> IDPRFPHHHPRPQSFWEARAKALESLLIEKGHLSSDASERVIKHYEHEL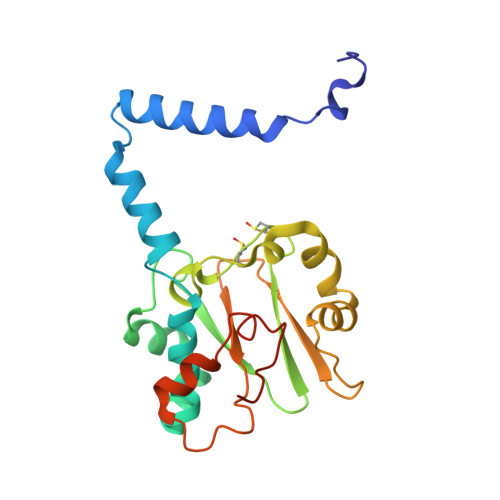GPMNGAKVVAKAWTDPAFKQRLLEDSETVLRELGYYGLQGEHIRVVENTDTVHNVVVCTLCSCYPWPLLGLPPSWYKEPAYRARVVKEPRQVLKEFGLDLPDSVEIRVWDSSSEIRFMVLPQRPEGTEGMTEEELAKLVTRDSMIGVAKIEPPKVTVG>MKYIIEHMEEGFSEWVILEYSQILREVGAENLILSSLPESTTEKDIPQRLLKLGLRWTTKDLKGINEDFKDLELLKDGRVCLLDPRATIDLQPEDATKFDYFVFGGILGDHPPRDRTKELKTAYPNLLISRRLGDKQMTTDTAIRTTQLIIKDRIAFEDIKFIDYPEFRFNKNEATEM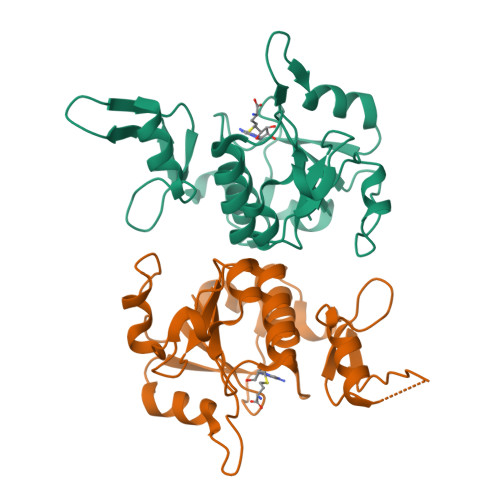PFRYVLDKEGKPILPEGMLDLIKKDSAQSLDDLLMLEHHHHHH[2x]DinG is another member of the XPD family, that appears to have a poorly defined role in DNA repair. The proteins comprise four domains; the helicase (HD1 and HD2), arch and FeS cluster domains. The FeS domain, that is inserted within the HD1 sequence, contains an iron-sulphur (FeS) cluster at its centre. Here, we present the crystal structures of two complexes of E. coli DinG; a binary complex bound to a ssDNA substrate, and a ternary complex with ssDNA and an ATP analogue (ADP•BeF3), that provide information about how these enzymes translocate on DNA.

The domain architecture of the ternary complex is similar to the binary complex, although there are changes in the relative orientations of the domains. Due to these changes, the protein now interacts with only ten bases of ssDNA. Although there are still three bases contacting HD1 and seven contacting HD2, there is no longer a base spanning the gap between the domains indicating that one of the domains must have slid along the ssDNA onto this base. Since the enzyme has 5’−3’ directionality, this would suggest it is the HD2 domain that has done the sliding. Consistent with this notion, the base at position +5 no longer stacks on base +6 (as seen in the binary complex) but instead would now clash with the P motif so becomes flipped up and over the strand to occupy the position taken by the +4 base in the binary complex. By contrast, the number of contacts between ssDNA and the HD2 domain is greater in the ternary complex. Upon ATP binding, a conformational change causes the HD2 motor domain to slide along ssDNA, while the HD1 domain retains a tight grip. The refined binary complex model contained one DinG molecule and one ssDNA molecule in the asymmetric unit, while the ternary complex model contained two DinG complexes in the asymmetric unit.

>[2x]MALTAALKAQIAAWYKALQEQIPDFIPRAPQRQMIADVAKTLAGEEGRHLAIEAPTGVGKTLSYLIPGIAIAREEQKTLVVSTANVALQDQIYSKDLPLLKKIIPDLKFTAAFGRGRYVCPRNLTALASTEPTQQDLLAFLDDELTPNNQEEQKRCAKLKGDLDTYKWDGLRDHTDIAIDDDLWRRLSTDKASCLNRNCYYYRECPFFVARREIQEAEVVVANHALVMAAMESEAVLPDPKNLLLVLDEGHHLPDVARDALEMSAEITAPWYRLQLDLFTKLVATCMEQFRPKTIPPLAIPERLNAHCEELYELIASLNNILNLYMPAGQEAEHRFAMGELPDEVLEICQRLAKLTEMLRGLAELFLNDLSEKTGSHDIVRLHRLILQMNRALGMFEAQSKLWRLASLAQSSGAPVTKWATREEREGQLHLWFHCVGIRVSDQLERLLWRSIPHIIVTSATLRSLNSFSRLQEMSGLKEKAGDRFVALDSPFNHCEQGKIVIPRMRVEPSIDNEEQHIAEMAAFFREQVESKKHLGMLVLFASGRAMQRFLDYVTDLRLMLLVQGDQPRYRLVELHRKRVANGERSVLVGLQSFAEGLDLKGDLLSQVHIHKIAFPPIDSPVVITEGEWLKSLNRYPFEVQSLPSASFNLIQQVGRLIRSHGCWGEVVIYDKRLLTKNYGKRLLDALPVFPIEQPEVPEGIVKKKEKTKSPRRRRR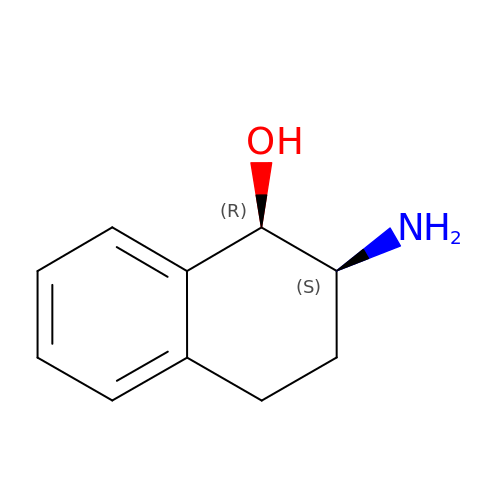CIS-(1R,2S)-2-AMINO-1,2,3,4-TETRAHYDRONAPHTHALEN-1-OL | C10 H13 N O | IIMSEFZOOYSTDO-VHSXEESVSA-N>[8x]MPLYVIDKPITLHILTQLRDKYTDQINFRKNLVRLGRILGYEISNTLDYEIVEVETPLGVKTKGVDITDLNNIVIINILRAAVPLVEGLLKAFPKARQGVIGASRVEV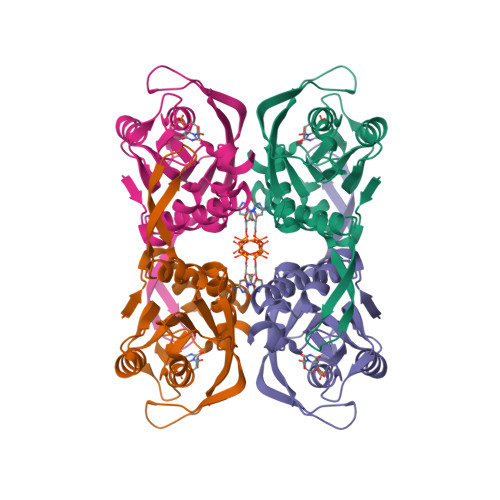DGKEVPKDMDVYIYYKKIPDIRAKVDNVIIADPMIATASTMLKVLEEVVKANPKRIYIVSIISSEYGVNKILSKYPFIYLFTVAIDPELNNKGYILPGLGDAGDRAFG>MSLSDDSTFGDATFVVLDFETTGLDPQVDEIIEIGAVKIQGGQIVDEYHTLIKPSREISRKSSEITGITQEMLENKRSIEEVLPE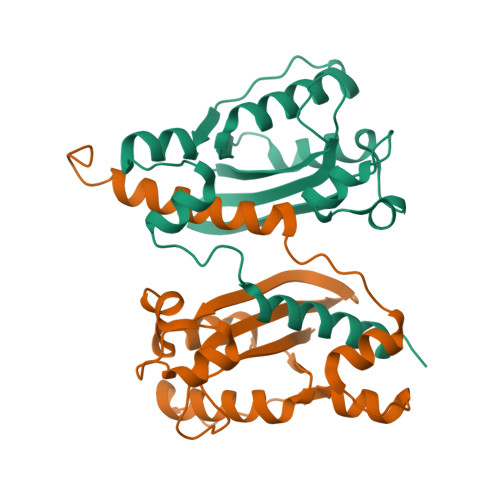FLGFLEDSIIVAHNANFDYRFLRLWIKKVMGLDWERPYIDTLALAKSLLKLRSYSLDSVVEKLGLGPFRHHRALDDARVTAQVFLRFVEMMKKEGHHHHHH[2x]>MLSKIKDSINSLRGITEKKLEKKDGTKYIMFGGKGGVGKTTMSAATGVYLAEKGLKVVIVSTDPAHSLRDIFEQEFGHEPTKVKGYDNLYVVEIDPQKAMEEYKEKLKAQIEENPFLGEMLEDQLEMAAL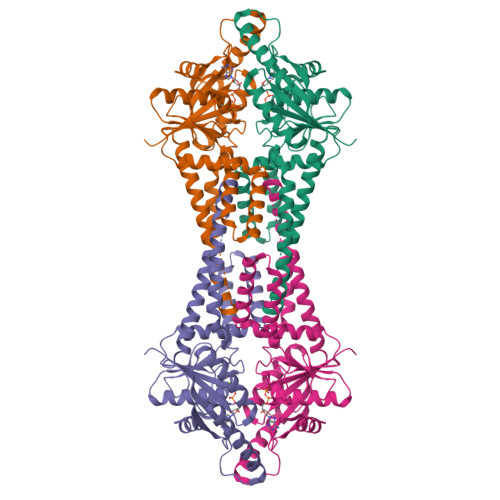SPGTDESAAFDVFLKYMDSNEFDVVIFDTAPTGHTLRFLGMPEVMDKYMTKLIKLRKQMSGFMKMMKKLLPFGGKDEDIDYDKMLEELEKMKERIVRARNILSDPERTAFRLVVIPEEMSILESERAMKALQKYGIPIDAVIVNQLIPEDVQCDFCRARRELQLKRLEMIKEKFGDKVIAYVPLLRTEAKGIETLKQIAKILYGEEEKEEQKIEQKVGQ[4x]>SMIFSVDKVRADFPVLSREVNGLPLAYLDSAASAQKPSQVIDAEAEFYRHGYAAVHRGIHTLSAQATEKMENVRKRASLFINARSAEELVFVRGTTEGINLVANSWGNSNVRAGDNIIISQMEHHANIVPWQMLCARVGAELRVIPLNPDGTLQLETLPTLFDEKTRLLAITHVSNVLGTENPLAEMITLAHQHGAKVLVDGAQAVMHHPVDVQALDCDFYVFSGHKLYGPTGIGILYVKEALLQEMPPWEGGGSMIATVSLSEGTTWTKAPWRFEAGTPNTGGIIGLGAALEYVSALGLNNIAEYEQNLMHYALSQLESVPDLTLYGPQNRLGVIAFNLGKHHAYDVGSFLDNYGIAVRTGHH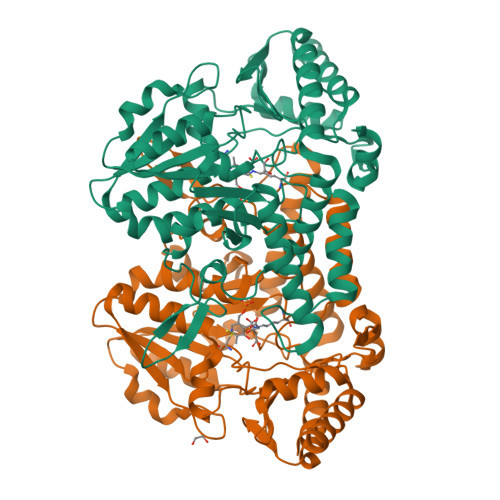CAMPLMAYYNVPAMCRASLAMYNTHEEVDRLVTGLQRIHRLLG[2x]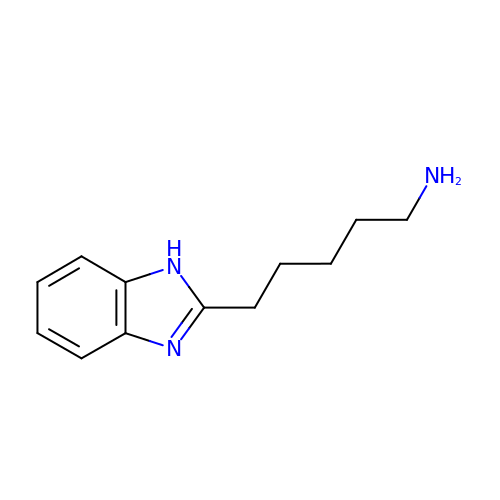5-(1H-benzimidazol-2-yl)pentan-1-amine | C12 H17 N3 | XTJRXHPNZGDOGE-UHFFFAOYSA-N> MDQSVSNVDKSSAFEYNKMIGHGINMGNALEAPVEGSWGVYIEDEYFKIIKERGFDSVRIPIRWSAHISEKYPYEIDKFFLDRVKHVVDVALKNDLVVIINCHHFEELYQAPDKYGPVLVEIWKQVAQAFKDYPDKLFFEIFNEPAQNLTPTKWNELYPKVLGEIRKTNPSRIVIIDVPNWSNYSYVRELKLVDDKNIIVSFHYYEPFNFTHQGAEWVSPTLPIGVKWEGKDWEVEQIRNHFKYVSEWAKKNNVPIFLGEFGAYSKADMESR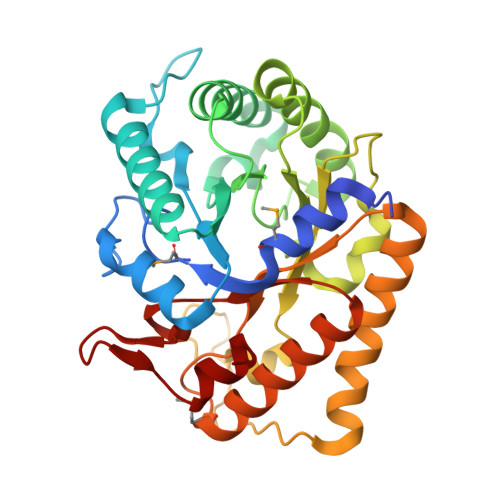VKWTKTVRRIAEEFGFSLAYWEFCAGFGLYDRWTKTWIEPLTTSALGK>NAQFLHTQVGRGLLGAVVNPLGEVTDKFAVTDNSEILYRPVDNAPPLYSERAAIEKPFLTGIKVIDSLLTCGEGQRMGIFASAGCGKTFLMNMLIEHSGADIYVIGLIGEAGREVTETVDYLKNSEKKSRCVLVYATSDYSSVDRCNAAYIATAIAEFFRTEGHKVALFIDSLTRYARAL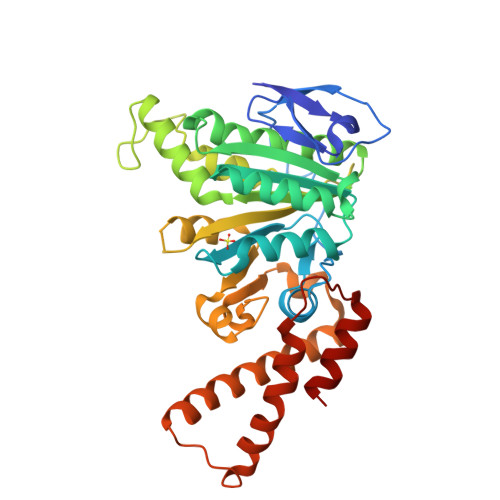RDVALAAGESPARRGYPVSVFDSLPRLLERPGKLKAGGSITAFYTVLLEDDDFADPLAEEVRSILDGHIYLSRNLAQKGQFPAIDSLKSISRVFTQVVDEKHRIMAAAFRELLSEIEELRTIIDFGEYKPGENASQDKIYNKISVVESFLKQDYRLGFTYEQTMELIGETIR[2x]>GSVESHPVLEKLKAAHSYNPKEFEWNLKSGRVFIIKSYSEDDIHRSIKYSIWCSTEHGNKRLDSAFRCMSSKGPVYLLFSVNGSGHFCGVAEMKSPVDYGTSAGVWSQDKWKGKFDVQWIFVKDVPNNQLRHIRLENNDNKPVTNSRDTQEVPLEKAKQVLKIISSYKHTTSIFDDFAHYEKRQAVVEVVRKERQSRNKQ[2x]

YTHDF proteins bind the N6-methyladenosine (m6A)-modified mRNAs, influencing their processing, stability, and translation. YTHDF proteins contain a hydrophobic pocket that accommodates the m6A embedded in the RRACH consensus sequence on mRNAs. The YTH domains of YTHDF1, DF2, and DF3 share a common fold with a central β-sheet surrounded by five α-helices. Three conserved tryptophan residues largely define the hydrophobic pocket involved in m6A binding.

YTH co-crystal structures were determined in complexes with compounds 7, 9, and 10. The complexes with compounds 9 and 10 are identical as the disulfide in compound 10 is reduced by Cys412 returning compound 9. Compound 9 establishes the disulfide bridge with Cys412, but the thiophenyl group is oriented in the opposite direction with respect to the ebselen selenophenol. The thiophenyl is again displaced with respect to ebselen and located similarly to compound 7. Instead, the morpholine ring assumes an opposite orientation, being directed toward the m6A site and occupying the position of Trp470 in the RNA-bound structure; it establishes van der Waals interactions with Tyr397 and Thr414. Interestingly, compound 10 interacts similarly to its reduced form compound 9. Interestingly, analogues 7 and 9 occupy the same specific small pocket of ebselen but the different substituents affect the binding poses of both the selenophenyl/thiophenyl headgroups and the tail moieties. In the YTH crystallographic structures presented here, either in complex with ebselen or its analogs, an aromatic ring occupies the small pocket defined by Asp401, Arg404, Ser405, Ile410, and Trp411, which then configures as the major hotspot. Binding poses of ebselen, compounds 7 and 9 diverge in the remaining regions and provide interesting growing vectors either toward the m6A pocket or residues lining it, as valuable determinants for increasing target specificity.>GPLGSDKALKMPASRYLTDMTLEEMSRDWFMLMPKQKVAGSLCIKMDQAIMDKTIILKANFSVIFDRLETLILLRAFTEEGAIVGEISPLPSLPGHTGEDVKNAIGVLIGGLEANDNTVRVTETIQR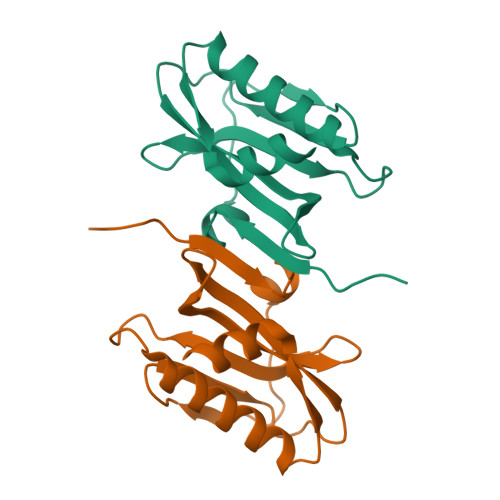FAWRNSDEDGRLPLPPNQKR[6x]>TGGRNSIRYSELAPLFDTTRVYLVDNKSTDVASLNYQNDHSNFLTTVIQNNDYSP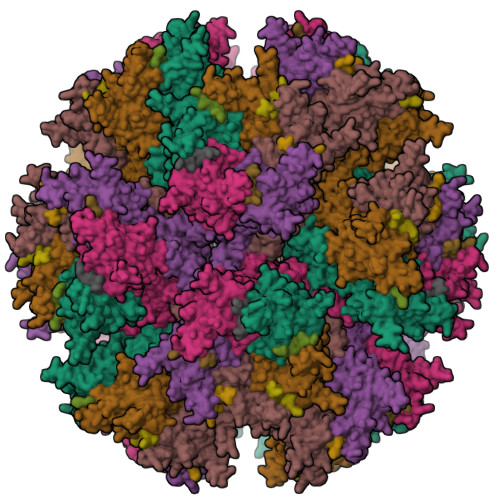GEASTQTINLDDRSHWGGDLKTILHTNMPNVNEFMFTNKFKARVMVSRSLTKDKQVELKYEWVEFTLPEGNYSETMTIDLMNNAIVEHYLKVGRQNGVLESDIGVKFDTRNFRLGFDPVTGLVMPGVYTNEAFHPDIILLPGCGVDFTHSRLSNLLGIRKRQPFQEGFRITYDDLEGGNIPALLDVDAYQASLKDDTEQGGDGAGGGNNSGSGAEENSNAAAAAMQPVEDMNDHAIRGDTFATRAEEKRAEAEAAAEAAAPAAQPEVEKPQKKPVIKPLTEDSKKRSYNLISNDSTFTQYRSWYLAYNYGDPQTGIRSWTLLCTPDVTCGSEQVYWSLPDMMQDPVTFRSTSQISNFPVVGAELLPVHSKSFYNDQAVYSQLIRQFTSLTHVFNRFPENQILARPPAPTITTVSENVPALTDHGTLPLRNSIGGVQRVTITDARRRTCPYVYKALGIVSPRVLSSRTF[5x];>[5x]MKRARPSGDTFNPVYPYDT> GPLGSPEFEDDLYRQSLEIISRYLREQATGSKDSKPLGEAGAAGRRALETLRRVGDGVQRNHETAFQGMLRKLD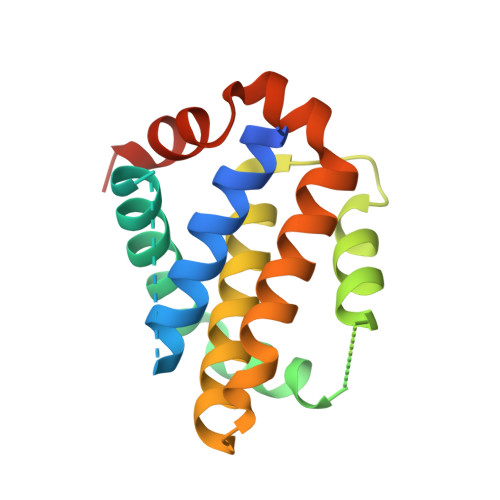IKNEGDVKSFSRVMVHVFKDGVTNWGRIVTLISFGAFVAKHLKSVNQESFIEPLAETITDVLVRTKRDWLVKQRGWDGFVEFFHVQDLEGG>[2x]SFSNFPISEETIKLLKGRGVTFLFPIQAKTFHHVYSGKDLIAQARTGTGKTFSFAIPLIEKLHGELQDRKRGRAPQVLVLAPTRELANQVSKDFSDITKKLSVACFYGGTPYGGQFERMRNGIDILVGTPGRIKDHIQNGKLDLTKLKHVVLDEVDQMLDMGFADQVEEILSVAYKKDSEDNPQTLLFSATCPHWVFNVAKKYMKSTYEQVDLIGKKTQKTAITVEHLAIKCHWTQRAAVIG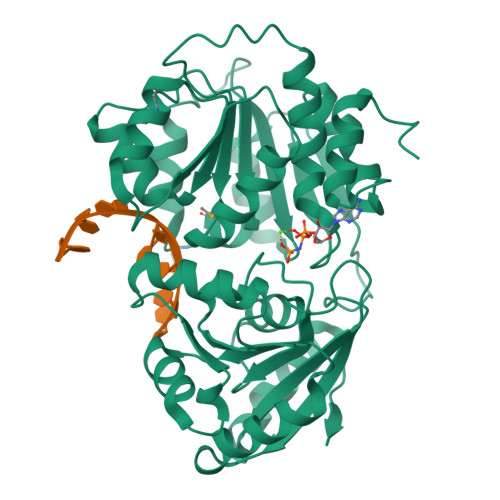DVIRVYSGHQGRTIIFCETKKEAQELSQNSAIKQDAQSLHGDIPQKQREITLKGFRNGSFGVLVATNVAARGLDIPEVDLVIQSSPPKDVESYIHRSGRTGRAGRTGVCICFYQHKEEYQLVQVEQKAGIKFKRI> SGLSITTPEQRIEKAKGETAYLPCKFTLSPEDQGPLDIEWLISPSDNQIVDQVIILYSGDKIYDNYYPDLKGRVHFTSNDVKSGDASINVTNLQLSDIGT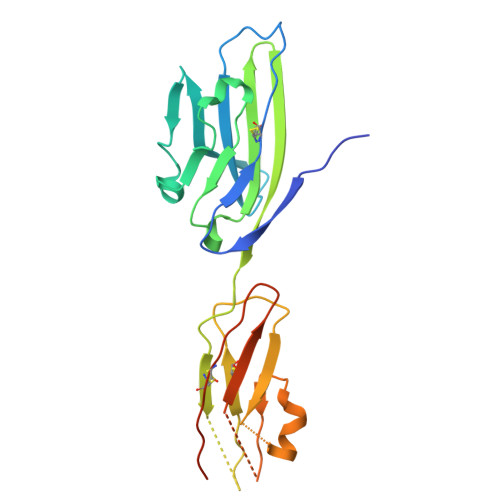YQCKVKKAPGVANKKFLLTVLVKPSGTRCFVDGSEEIGNDFKLKCEPKEGSLPLQFEWQKLSDSQTMPTPWLAEMTSPVISVKNASSEYSGTYSCTVQNRVGSDQCMLRLDVVPPSNRAHHHHHH> MALKTKIIVQQILNIDDTTTTASKYPKYTVVLGNSISSITAGELTAAVEASAGSAAAAKGSEIAAKESELNAKDSENEAAISAGASEESASQSAASAAESERQAGLSKGSADNSAASAQESEGFRDSAELAAQNAEQSRLLAEQAKTAAQQAQTAAEAAKTGAETAKDGADAAATTAGEHAAAARQSELNAKISETNAAGSATEAGDKAIDATTEADRAKAEADRATQIVDSKLDKVDISGFIKVYKTKAEADADVVNRVLDEKVLVWNQTNSKYGWYKVAGTAETPVLELVETEQKLTSVNNVRADDAGNVQITLPGGNPSLWLGEVTWFPYDKDSGVGYPGVLPADGREVLRVDYPDTWEAIEAGLIPSVSEAEWQAGASLYFSTGDGSTTFRLPDMMQGQAFRAPT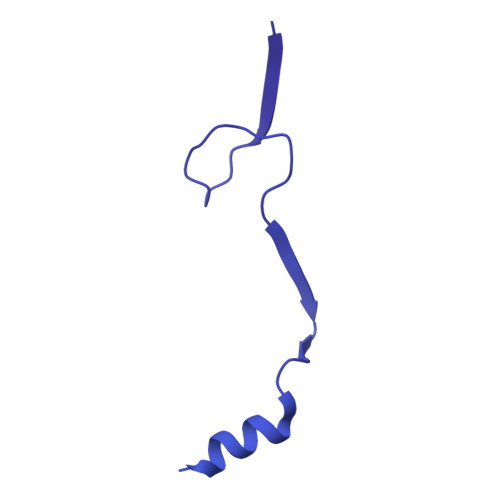KGEEDAGVIKDQIPYVVTVNGISPDAITGNVEIDTSLQGTVSINQGGTGATTKEDARIALELYSTTEVDSALADKADIATTYTKTEVDSALADKADIATTYTKVEVDSALADAKTQSDTDYLLKANNLSDLADRAAAWLNVRPIGSTPLAGDPVGDYDAVTKRWVENKINTGTVGPTMNGVMNYGVGDFHLRDSRAYIQPYEVVSDGQLLNRADWPELWAYAQMLSPISDADWLADPTKRGQYSLGDGSTTFRVPDRNGVQTGSISALFGRGDGGASSTGGTILDSAAPNITGSFGRLVYASTGTIYEANTGTGAFSAVLSQAKYKRLSEISAADGTAATYPSGFEFFASNSSPVYGRGSTEVRPKAFTGVWVIRASGGFVAANTSWSVINGDATRPADGTTADGGEIISRYNVNGVREAQMSWRIRAQIGAEHYARLNVYNATANRTAVYDFNDLGTFSAENLHSKGAIYSDGNLTIQNQGWPGINFKSNRYNTPATQIGGSTIIEVSGTDGNVSGVNLIRRRGDGNQAGQIIVSFPTTGGAIALQGTSGIEYKKDVTDADAQEAMDRINGQRLVNFVYKDDEQERVRFGVIAEEAELIAPQYIKHNQVSYEDILDEEGNKIGEKTRDRPSVDVNPIVMDLMGCVQALNAKIAALEARIAELESKE> GSKPGDSYNTPWGKVIIN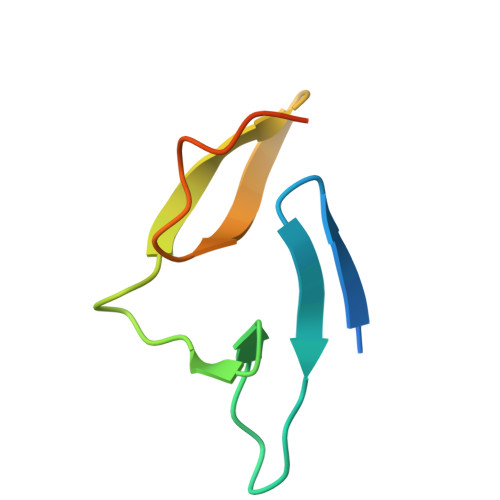AAGQPTMNGTVMTADNSSMVPYGRGFTRVLNSLVNNPVSHHHHHH>[2x]MDMGISGKVAVITGSSSGIGLAIAEGFAKEGAHIVLVARQVDRLHEAARSLKEKFGVRVLEVAVDVATPEGVDAVVESVRSSFGGADILVNNAGTGSNETI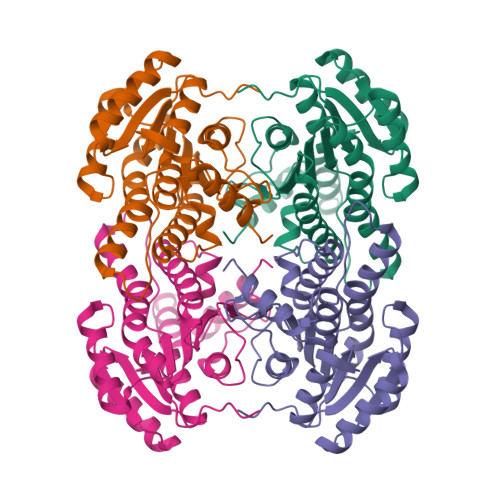MEAADEKWQFYWELHVMAAVRLARGLVPGMRARGGGAIIHNASICAVQPLWYEPIYNVTKAALMMFSKTLATEVIKDNIRVNCINPGLILTPDWIKTAKELTKDNGGDWKGYLQSVADEHAPIKRFASPEELANFFVFLCSERATYSVGSAYFVDGGMLKTL hexyl(octoxy)phosphinic 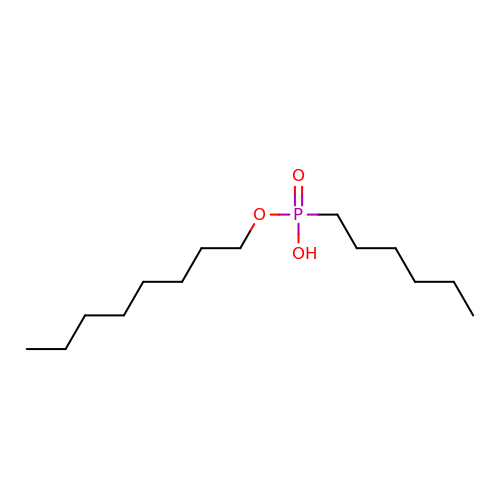acid | C14 H31 O3 P | ITXAFDXPCLYZIG-UHFFFAOYSA-N> MEKRINKIRKKLSADNATKP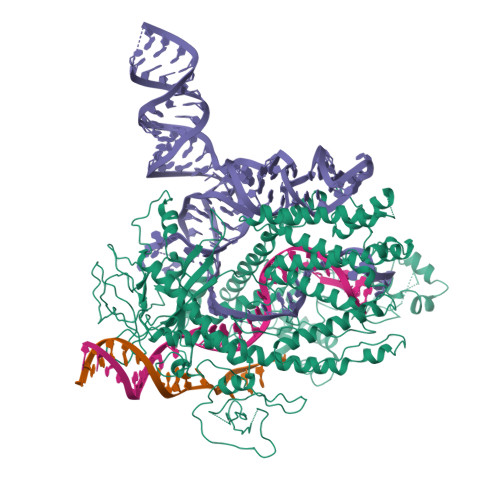VSRSGPMKTLLVRVMTDDLKKRLEKRRKKPEVMPQVISNNAANNLRMLLDDYTKMKEAILQVYWQEFKDDHVGLMCKFAQPASXXXXXXXXXXXXXXXXXXXXXXXXXXXXXXXXXXXXXXXXXXXXXXXXXXXXXXXXXXXXXXXXXXXXXXXXXXXXXXXXXXGKFGQRALDFYSIHVTKESTHPVKPLAQIAGNRYASGPVGKALSDACMGTIASFLSKYQDIIIEHQKVVKGNQKRLESLRELAGKENLEYPSVTLPPQPHTKEGVDAYNEVIARVRMWVNLNLWQKLKLSRDDAKPLLRLKGFPSFPVVERRENEVDWWNTINEVKKLIDAKRDMGRVFWSGVTAEKRNTILEGYNYLPNENDHKKREGSLENPKKPAKRQFGDLLLYLEKKYAGDWGKVFDEAWERIDKKIAGLTSHIEREEARNAEDAQSKAVLTDWLRAKASFVLERLKEMDEKEFYACEIQLQKWYGDLRGNPFAVEAENRVVDISGFSIGSDGHSIQYRNLLAWKYLENGKREFYLLMNYGKKGRIRFTDGTDIKKSGKWQGLLYGGGKAKVIDLTFDPDDEQLIILPLAFGTRQGREFIWNDLLSLETGLIKLANGRVIEKTIYNKKIGRDEPALFVALTFERREVVDPSNIKPVNLIGVARGENIPAVIALTDPEGCPLPEFKDSSGGPTDILRIGEGYKEKQRAIQAAKEVEQRRAGGYSRKFASKSRNLADDMVRNSARDLFYHAVTHDAVLVFANLSRGFGRQGKRTFMTERQYTKMEDWLTAKLAYEGLTSKTYLSKTLAQYTSKTCSNCGFXXXXXXXXXXXXXXXXXXXXXXXXXXXXXXXXXXXXXXXXXXXXXXXXXXXXXXXXXXXXXXXXXXXXXXXXXXXXXXXXXXXXRFSHRPVQEQFVCLDCGHEVHAAEQAALNIARSWLFLNSNSTEFKSYKSGKQPFVGAWQAFYKRRLKEVWKPNA>[8x]MMVISEKVRKALNDQLNREIYSSYLYLSMATYFDAEGFKGFAHWMKKQAQEELTHAMKFYEYIYARGGRVELEAIEKPPSNWNGIKDAFEAALKHEEFVTQSIYN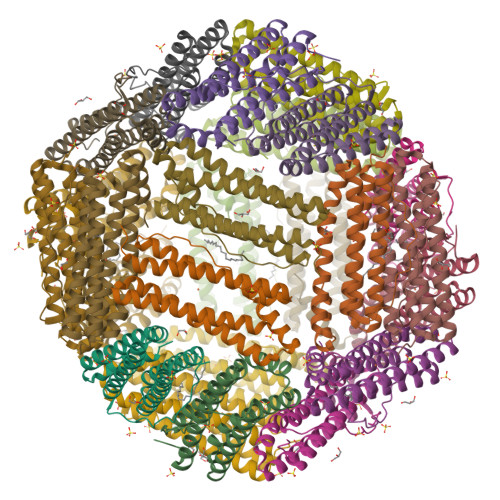ILELASEEKDHATVSFLKWFVDEQVEEEDQVREILDLLEKANGQMSVIFQLDRYLGQRE>[2x]MSLRVIDTHCDALYKLQAGKGKYTFQDAEELDVNFERLIEAKMLLQGFAIFLDEDIPVEHKWKKAVEQVNIFKQHVLHKGGIIHHVKKWCDLENLPEDKIGAMLTLEGIEPIGRDLDKLTQLLDGGVLSVGLTWNNANLAADGIMEERGAGLTRFGKDIIHLLNERKVFTDVSHLSVKAFWETLEQAEFV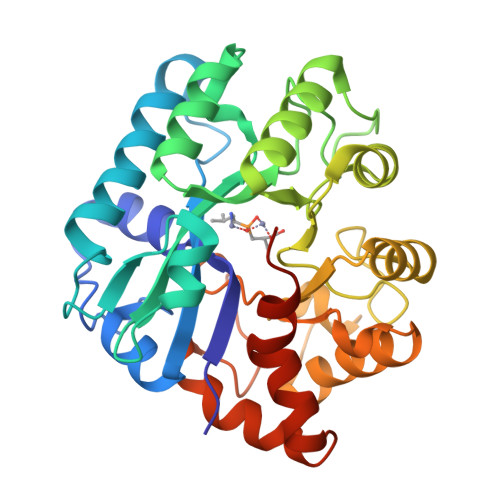IASHSNAKAICSHPRNLDDEQIKAMIEHDAMIHVVFYPLFTTNNGVADTEDVIRHIDHICELGGLKNIGFGSDFDGIPDHVKGLEHVGKYQSFLETLEKHYTKEEIEGFASRNFLNHLPKEGHHHHHH> ATLAQDVIDRFDVSRPEL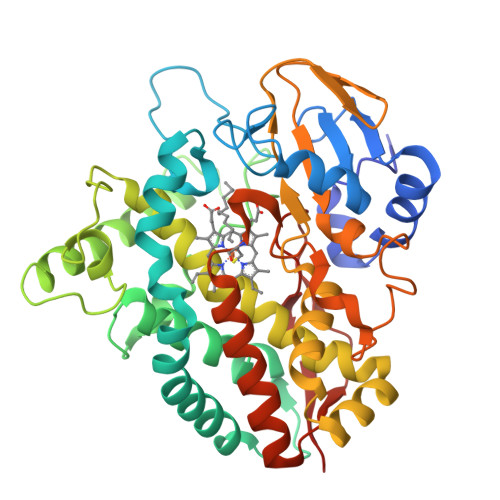YRDDLWQAPFRELRATAPVHRVEHSDFGPYWSVSSYKPIITVESLPDLYSSAGGITLADFIENNPTDVRMPMFIAMDRPKHTGQRRTVAPAFTPSEMVRMSDNIRMRTAEVLDSLEWNTPFDWVDTVSVELTTQMLAILFDFPWEERRKLTFWSDWAGDIELVKNEELRLERLRHMYECGGYFQNLWNAKIGKPPTPDLISMMIHSDAMAEMDQMEFLGNLILLIVGGNDTTRNTMSAVAYGLDLFPDQRAKLEADPSMIPNTVQEIIRWQTPLAHMRRTATVDSELEGQQIKAGDKLALWYISANRDESVFENADRIIVDRPNARRHLAFGHGIHRCVGARLAELQIAVLLEEMAKRRMRVNVLGEPERVAACFVHGYRKLPVEISRY Most HAdVs are equipped with twelve protruding fiber proteins that mediate attachment to host cell receptor molecules. Unlike most other HAdVs, this virus contains two different fiber proteins, a long and a short one, a feature shared only with the two members of species HAdV-F (HAdV-40 and -41). We find that the long fiber binds to a protein-based receptor known as the coxsackievirus and adenovirus receptor (CAR), and that the short fiber binds to glycoproteins that contain sialic acid-capped glycans. Similar to all other known AdV fiber knob structures the 52SFK has a nine-stranded antiparallel β-sandwich fold and forms a stable trimer in solution.

In order to define the interactions of the HAdV-52 fiber with sialic acid, we solved the crystal structure of 52SFK in complex with 2-O-methyl-sialic acid (a stereochemically uniform analogue of sialic acid) at a resolution of 1.65 Å. The three shallow sialic acid binding sites of 52SFK are formed at the contact site of two neighboring monomers by the EG and GH loops at the side of the short fiber knob domain. Two of the three binding sites are partially blocked by crystal contacts, and therefore the structure contains only one fully occupied sialic acid, while a second sialic acid is visible with partial occupancy in one of the two partially blocked binding sites. The bound 2-O-methyl-sialic acid is well defined by electron density and engages the 52SFK mainly through contacts between the sugar’s carboxylate group and the side chains of R316 and N318. The bidentate salt bridge formed by R316 is a prominent binding motif among glycan binding viruses. In addition, the backbone carbonyl oxygens of R316, G317, and G303 form hydrogen bonds with the sialic acid O4, N-acetyl and glycerol-like functions, respectively. The tripeptide R316-G317-N318 located on the GH loop forms a hook-shaped motif (RGN motif) that is contributing most of the interactions, and that therefore largely defines the specificity of SFK52 for sialic acid. Mutating either R316 or N318 to alanine, replacing the R316 side chain with a negatively charged glutamate, or introducing a steric clash (and a polar clash, introducing a charge) at position 308 (N308E) all abolished the attachment of 52SFK to Pro-5 and A549 cells. The sugar’s O2 function, to which additional sugars would be attached in a glycan chain, is pointing away from the protein and towards the tip of the knob, suggesting that more complex glycan receptors that bind the knob with their sialic acid caps would have to face towards the capsid in order to be bound by the virus. The mode of interaction between 52SFK and its sialylated receptors is fundamentally different, both in location on the protein and in contacts formed to the ligand, from the known interactions between HAdV-37 fiber knob and sialic acid.

>[3x]MRGSHHHHHHGSGSGSGIEGRPYNGTGSRFNSSGAIAFGIQTLWTPPTSNPNCTVYTESDSLLSLCLTKCGAHVLGSVSLTGVAGTMTNMAETSLAIEFTFDDTGKLLHSPLVNNTFSIRQGDSPASNPTYNALAFMPNSTLYARGGSGEPRNNYYVQTYLRGNVQRPITLTVTFNSAATGYSLSFKWTAVVREKFAAPATSFCYITEQ>[2x]MGSSHHHHHHSQDP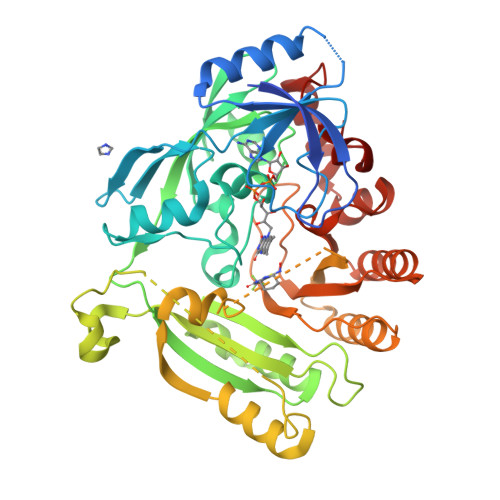MLSVGATTTATRLTGWGRTAPSVANVLRTPDAEMIVKAVARVAESGGGRGAIARGLGRSYGDNAQNGGGLVIDMTPLNTIHSIDADTKLVDIDAGVNLDQLMKAALPFGLWVPVLPGTRQVTVGGAIACDIHGKNHHSAGSFGNHVRSMDLLTADGEIRHLTPTGEDAELFWATVGGNGLTGIIMRATIEMTPTSTAYFIADGDVTASLDETIALHSDGSEARYTYSSAWFDAISAPPKLGRAAVSRGRLATVEQLPAKLRSEPLKFDAPQLLTLPDVFPNGLANKYTFGPIGELWYRKSGTYRGKVQNLTQFYHPLDMFGEWNRAYGPAGFLQYQFVIPTEAVDEFKKIIGVIQASGHYSFLNVFKLFGPRNQAPLSFPIPGWNICVDFPIKDGLGKFVSELDRRVLEFGGRLYTAKDSRTTAETFHAMYPRVDEWISVRRKVDPLRVFASDMARRLELL> SVLLITELPEDGCTEEDVRKLFQPFGKVNDVLIVPYRKEAYLEMEFKEAITAIMKYIETTP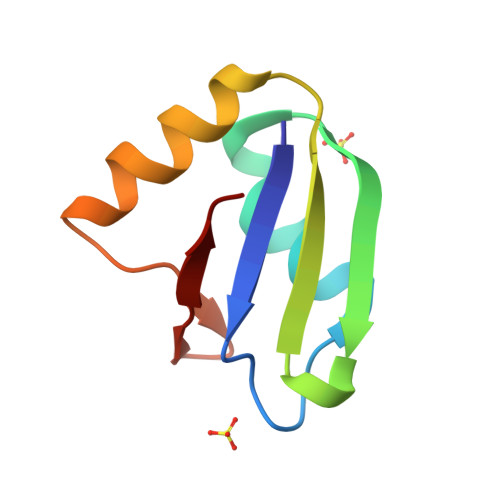LTIKGKSVKICVP1-PHENYLHYDRAZINE | 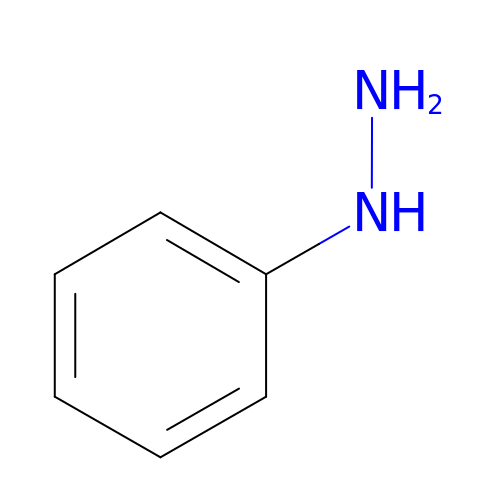C6 H8 N2 | HKOOXMFOFWEVGF-UHFFFAOYSA-N>[2x]GSHMADKELKFLVVDDFSTMRRIVRNLLKELGFN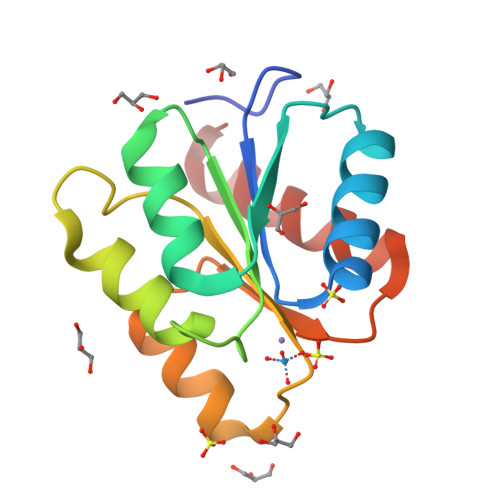NVEEAEDGVDALNKLQAGGYGFVISDWDMPNMDGLELLKTIRADGAMSALPVLMVTARAKKENIIAAAQAGASGYVVKPFTAATLEEKLNKIFEKLGM> SNATPAPREAEAAALLAATVADPW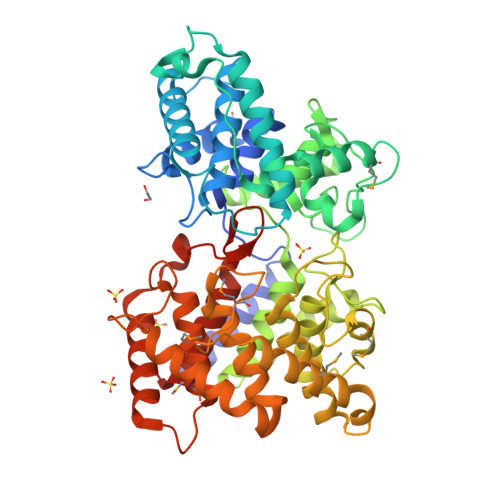GLVAPSVYDTARLVSLAPWLDGHRERLGYLAKEQNQDGSWGAPDGYGLVPTLSAVEALLTELARTDSGAPHLSPDDLAAACADGLGALRDGLLAGPVPDTIGVEFVAPSLLADINTRLAALTEQAPGKLGAWSGTTLTSPAPDLDGALLAGVREMTEQAPLPEKLWHTLEAVTRDGTRGARPHEGAPPHNGSVGCSPAATAAWLGAAPDPAAPGVAYLRDVQARFGGPVPSITPIVYFEQAWVLNSLAASGLRYEAPAALLDSLEAGLTDEGIAAAPGLPSDSDDTAAVLFALAQHGRTHRPDSLMHFRRDGYFSCFGVERTPSTSTNAHILEALGHHVTVRPDDAGRYGAEIRMISDWLLDNQLPDGSWMDKWHASPYYATACCALALAEFGGPSARAAVDRAAAWALATQRADGSWGRWQGTTEETAYMVQLLMRTRTPGSPGTVARSAARGCDALLAHDDPASYPGLWHDKDIYAPVTVIRAARLAALALGGAASA>[2x]MAPKTQKRAAAKFYQEDIVQRKDDSNTFGVILRCWQDAEETPPAGDHIDPLMRPLVQGEVGVSYFPKPMREIVPEDTLELVDRLYQPGDLLKRSVDDVRSGVVTRTHVKGRLEHAVSSFSLPGWKSMEEIESAVEIDMGEYVIYNDWVGQVVEMFDESLVEVPGGTLVRLPELSARLAVGEKGQDILPQPVGSVTGILGFLLGGTRPSDRDTVISVKHTVLAVAWLAINQSLSPEEAQGKPRPQRYWYGEDLGKLTTITRK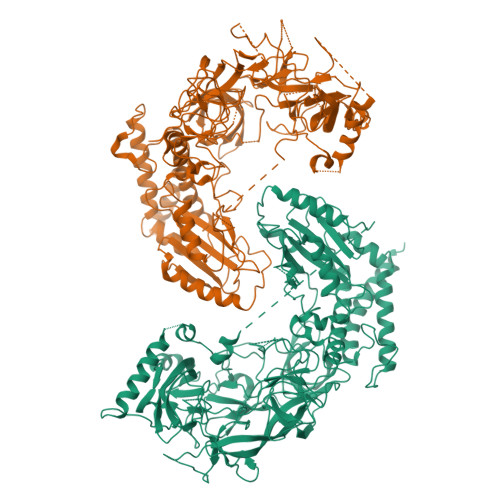AEEAMRVGDRVKLKNTRDGPVTRHGRPLEGVIEVDTLVVQETRTSVDVLWQDGTRETMDVKQTVPYLNPDEYDCWPGDHVLWKTEDHKRHVVVQSVNAQDRTAYVRVVETGAVELASVLELDPHGSGDWSPLAPANDGLGVRRGDFVFIHREGTTNGARAPMVPRIGEVEEWVREAPTLGPNGQIGGWRSEMTELGSRIAEQRGKEGSVDEVPLKQAQKGDTSLNWFGEVLDLRLDGTIEVILPSADTIVVPLERLTRLYDSVEQLEDLWGDDEGTVEDEDDVEVWEMDQDGHWVEGTMDGDDDEWESADEELDPADSMDVEGGEWSPSTDTVTIPPPINGETPMAVDSALPPETQSSAATQSPSPHPPKEAGDVEDGPWKRFEVLPSAPVDHAFYNTPPAQHTRQFMARMSKEYKALQSSLPDSILVRAYEDRTDLLRSLIIGPENTPYEDAPFVIDWMLDANFPQTPPIAHFLSWTNGNGRVNPNLYEEGKVCLSILGTWAGDKSESWSASRSSLLQALVSIQGLVLVKEPWFCEPAYEKLRGTEDGIVNSRLYNEKAYVLSRGFVRRALEIPLGGLEEELRWFYHTSGKLRKVLGDARALIVKSTATQGDAEVPEADRERAVPRLSSGGIIALERTLGKLQALQDAQTATEANAADGAKAKAER Here, we identify five lycibarbarspermidine glycosyltransferases, LbUGT1-5, which are the first phenolamide-type glycosyltransferases and catalyze regioselective glycosylation of dicaffeoylspermidines to form structurally diverse lycibarbarspermidines in wolfberry. LbUGT1 and LbUGT3 are the first phenolamide-type glycosyltransferases with crystal structures, and both exhibit a canonical GT-B fold consisting of two Rossmann-like fold (β/α/β) domains in the N and C-termini. The N-terminal domain (residues 1–242 and 467–485 in LbUGT1, residues 1–246 and 464–482 in LbUGT3) is mainly involved in the binding of sugar acceptor, while the C-terminal domain (residues 243–466 in LbGT1, residues 247–463 in LbGT3) is responsible for the binding of sugar donor.

LbUGT1 is the only UGT that can recognize both the dihydrocaffeoyl and caffeoyl moieties, selectively catalyzing a sugar transfer to the 3’-OH of the caffeoyl group and the 4”-OH of the dihydrocaffeoyl group. In order to elucidate the molecular mechanism, the acceptor substrate 1 was docked into LbUGT1 structure, the MD simulations revealed the two active binding modes, corresponding to 4”-O-glycosylation (mode 1) and 3’-O-glycosylation (mode 2), respectively, which were verified by the small d1 and d2 values during the 50 ns simulations (left). In addition, both binding modes showed several negatively charged residues, i.e., aspartic acids and glutamic acids (E83, D197, D416, E418), reside near the positively charged N5 of the substrate 1 (protonated in physiological environment). These residues may stabilize the conformation of the substrate through electrostatic or salt bridge interactions, and thus could play a crucial role in recognizing the spermidine unit of the substrate. Comparisons of the two binding modes revealed that the residue interactions are essentially identical except for Y389, which forms a hydrogen bond with the 3”-OH of the acceptor substrate in binding mode 1, but not in binding mode 2, suggesting that Y389 might play an important role in stabilizing binding mode 1 for the 4”-OH glycosylation of the dihydrocaffeoyl moiety. In contrast, the mutant Y389A remarkably changed its regioselectivity by eliminating its activity towards the 4”-OH but enhancing its activity at the 3’-OH. Additionally, the mutation of Y389 to F also showed increased 3’-O glycosylation activity and impaired 4”-O glycosylation activity, indicating the important role of the OH group of Y389 in the 4”-O glycosylation activity. Though both LbUGT1 and LbUGT3 first catalyze the 3’-OH glycosylation of the caffeoyl group, LbUGT3 can further catalyze the 4’-OH glycosylation on the same side of 2 to form an unusual ortho-diglucosylated product, while LbUGT1 needs to rotate the mono-glucosylated product for a sugar transfer to the 3”-OH on the opposite side.

> GSEFELRRQALTTKAELVFIPSPGAGHLISAIEIAKLILNRDERLCISVLIMKLPMDFGVQSYVASLSSSPRLQFVDITLDEKTVAGLLKNKESFFTDFIQGHKPKVKDFIHNTSFSKSGSGFSRLAGFVLDMFCTSMIDVASEFSVPSYIFLTSNAAFLALCYHFESLKKEHHIDTSKYKDSDEELTIPGFKNPYPGKFLPRLTTDQTTATTLFFDSVTRFKETKGIMVNTFAELEPFALQSLLVPKIYPVGPVVNFKEGGHGRNSESETESIIKWLDDQPESSVVFLCFGSMGSFDAEQIEEIAVALECSGHRFLWSLRRPPPKGKMELPSNYEDFQEVLPEGFIERTNGVGKVIGWAPQVAVLSHPAVGGFVSHCGWNSVLESLCFGVPIGAWPQYAEQQMNAFELVKQLGLAVEIRMDYFKDFEGKHGPVEIVTAKEIASGIRQLMADGEENEIRKRAKEMKEKSSAAMKEGGSSYASLGLLIEDVISNIS>KESRAKKFQRQHMDSDSSPSSSSTYCNLMMCCRKMTQGRCK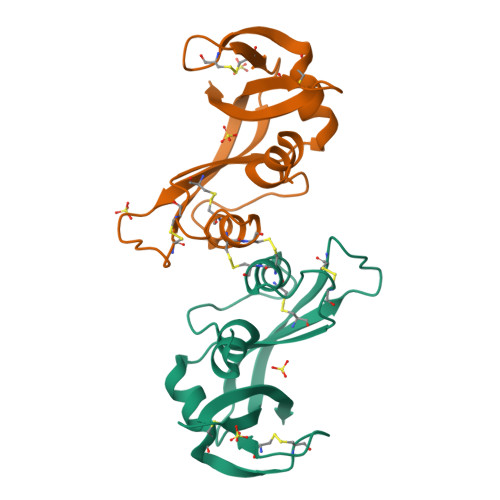PVNTFVHEPLVDVQNVCFQEKVTCKNGQGNCYKSNSSMHITDCRLTNGSRYPNCAYRTSPKERHIIVACGGSPYVPVHFDASVE[2x]> AKGALQELGAG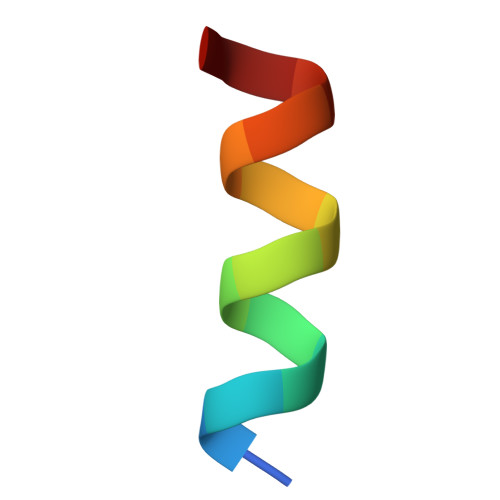LTA>XSLSDKDKAAVRALWSKIGKSSDAIGNDALSRMIVVYPQTKIYFSHWPDVTPGSPNIKAHGKKVMGGIALAVSKIDDLKTGLMELSEQHAYKLRVDPSNFKILNHCILVVISTMFPKEFTPEAHVSLDKFLSGVALALAERYR[2x];>VEWTDKERSIISDIFSHMDYDDIGPKALSRCLVVYPWTQRYFSGFGNLYNAEGIMSNANVAAHGIKVLHGLDRGMKNMDNIADAYTDLSTLHSEKLHVDPDNFKLLSDCITIVLAAKMGHA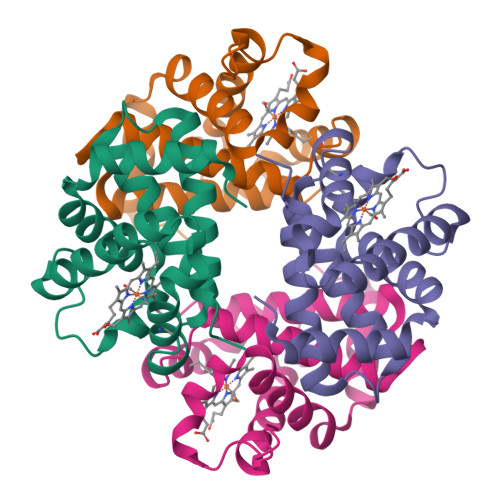FTAETQGAFQKFLAAVVSALGKQYH[2x]>GFLHVGAQLGTELFIVRQLLQIVKQKTNQNSVDTTLKFTLSALWNLTDESPTTCRHFIENQGLELFMRVLESFPTESSIQQKVLGLLNNIAEVQELHSELMWKDFIDHISSLLHSVEVEVSYFAAGIIAHLISRGEQAWTLSRSQRNSLLDDLHSAILKWPTPECEMVAYRSFNPFFPLLGCFTTPGVQLWAVWAMQHVCSKNPSRYCSMLIEEGGLQHLYNIKDHEHTDPH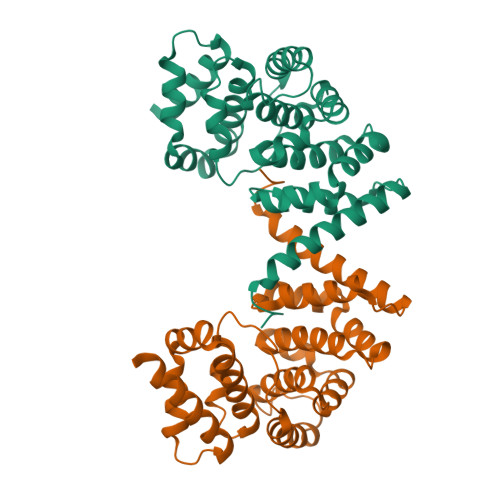VQQIAVAILDSLEKHIVR[2x]>[5x]QDMVSPPPPIADEPLTVNTGIYLIECYSLDDKAETFKVNAFLSLSWKDRRLAFDPVRSGVRVKTYEPEAIWIPEIRFVNVENARDADVVDISVSPDGTVQYLERFSARVLSPLDFRRYPFDSQTLHIYLIVRSVDTRNIVLAVDLEKVGKNDDVFLTGWDIESFTAVVKPANFALEDRLESKLDYQLRISRQYFSYIPNIILPMLFILFISWTAFWSTSYEANVTLVVSTLIAHIAFNILVETNL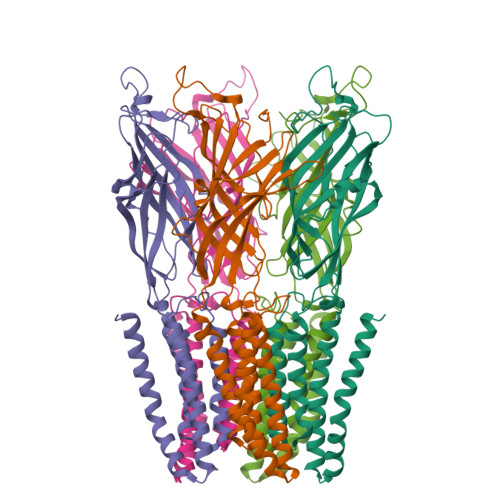GKTPYMTYTGAIIFMIYLFYFVAVIEVTVQHYLKVESQPARAASITRASRIAFPVVFLLANIILAFLFFGF>GSHMASMETLNDLVTRLEHSHPNSSLLKDLSLIQGNEQYNYIKWGDLSNSQNLNELVFQYEKAPYPSITCGILTYNEERCIKRCLDSLGSQFDEILVLDSHSTDNTTKIINRDFPMVKVIYEPWIDDFSFHRNKLISLTSSEWIYYIDADNYCVDSTNKFKRVAKLIQFLSIDCIISPMIKEHIGHVYTDNRKMFSVKKGIQFKGKVHEEPINADGSIPQNITVDIMICHDGYDPEVINLSEKNDRNIKLTRQMMEEEPSNPKWLYFYARELHYASEDTHIIETLLIKAIDLYKQSTYKRYQPEAILLLCSILFQKRQIRKLNEYLDLLEELQPLCSDVNYYRSLILFYDIRLKTGKLLDTLKSSELENNKYSFIDSSKDHIKALLIELYCSIDDWEGAFTLFDELQSTE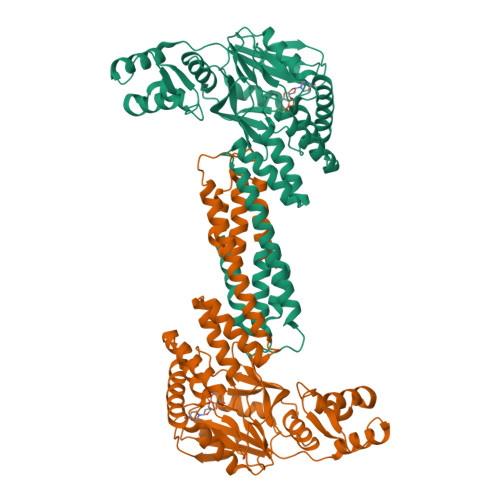ARNKFLRRVKTINTHISKKI[2x]The first committed reaction in grindelic acid biosynthesis is the transformation of the core diterpenoid precursor geranylgeranyl diphosphate (GGPP) into the bicyclic intermediate 7,13-copalyl diphosphate (7,13-CPP) catalyzed by the class II diterpene synthase (diTPS) Grindelia robusta TPS2 (GrTPS2). GrTPS2 is mechanistically closely related to other class II diTPS enzymes that facilitate the protonation-dependent cyclization of GGPP to form a range of CPP intermediates via a common labda-13-en-8-yl+ diphosphate intermediate. All class II diTPS share a common three-domain (γβα) fold with the active site being formed by the N-terminal γ and β domains. A conserved catalytic DxDD motif controls the general acid-base mechanism to bring about the cyclization of GGPP with the middle Asp residue functioning as the general acid.

The GrTPS2 crystal structure adopts the conserved three-domain fold of class II diterpene synthases featuring a functional active site in the γβ-domain and a vestigial ɑ-domain. The N-terminal segment (residues 1–18) and a short region of the J-K loop in the α-domain (residues 563–566) are disordered in the GrTPS2 structure. Consistent with other class II diTPSs, the C-terminal α-domain lacks helices α1 and G1 and helices D, F, H, and I are shorter as compared to class I diTPSs resulting in a non-functional class I active site. The GrTPS2 class II active site is formed by the γ- and β-domains, which adopt the typical ɑ-barrel structure and closely resemble the AtCPS active site. AtCPS E211, predicted to be involved in substrate binding and the catalytic DIDD motif, including D325 as the general acid functioning in substrate protonation, is conserved in GrTPS2 (E157) and situated at the bottom of the active site cavity. By contrast, a His-Asn dyad, previously shown to be important for catalytic specificity in AtCPS and other ent-CPP synthases, is replaced with Tyr (Y209) and Thr (T268) residues located at the top of the active site. The respective GrTPS2 residues, namely D449, R286, R283, and D282, are conserved in GrTPS2 and coordinate several water molecules. The presence of a solvent channel in GrTPS2 is shown to connect the catalytic DIDD motif with bulk solvent similar to AtCPS. While the removal of a larger side chain through Ala substitution resulted in a nearly complete loss of function, exchange to His or Phe showed activity loss to a lesser extent and increased production of 8,13-CPP, suggesting that the hydroxyl group of Y457 and presence of an aromatic ring in this position make an important contribution to directing catalysis toward deprotonation of labda-13-en-8-yl+ at the endocyclic C-7 methylene to form 7,13-CPP.

> MCKAIYNPEKGLLKHSDLQLEDDKYSDLQLVDEKHTIKRSVESIKSALSLVDDGDLTLSAYDTAWVALIEDVNGRSGFPQFPSCLQWIVSQQLPDGSWGEPLMFLAFDRLLNTLASVVALTKWNIRPDICQKGMKYVLENLNKLVDEKEEHMTPGFELLFPKLIELAQKLDIKMPMDSPALKELYARRDTKLAKIPKKIFHKMPTILLYSLEGMNDLEWDKLLKLKSENGSFLCSPAATAFAFMETKDQDCLAYLTDLVAKFNGGVPTFYPTDMYEQIWIVDRLQRLGIAHYFSSEINNFVDHIYRYWDQKGISFARKCNLPDIDDTAMGFRVLRTHGYQVSSDVFQHFEKDGQFYCYWGQTAEAVTVMFNLYRASQVLFPGEKILDNAKKFAHNFLTEKVATNQVFDKWIITKDILGEVQYALDVPWYASLPRLEARYYLDQYAGDGDVWIAKTLYRLKYVSNNEYLETAKLDYNHCQKIHKLEWSYIQKWFLDLKIEESINTRTLWSYYQAAASIFHPERYNERLAWAKTNVLVDTITTFFSKQQMSKDDIQGFVNQLTNTENQQTYGKMSHMLIDALNETLKHISMKARETHGIDIYPHLQSSWKKWLLSCMNGPNVAGVAELIVETINLTSGRSFSNDLLSHPQYKQITSITNDLCHQLCSKGNRAIGSEIESKMQELVQLVFSDSSDGLDPDVKKTYLVVAKSFYYMAYFDAKTIDSHINKVLFEMVV N-[(1R,2R)-2-[4-(2-methoxyphenyl)piperazin-1-yl]cyclohexyl]benzenesulfonamide | C23 H31 N3 O3 S | 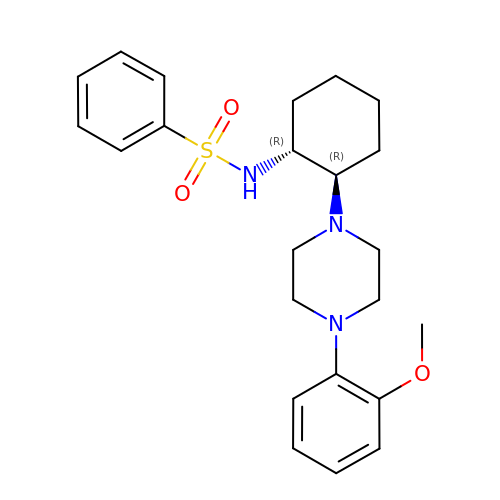OVTXOMMQHRIKGL-NHCUHLMSSA-N> GPLGSEILRHSMDPATFTFNFNNEPWVRGRHETYLCYEVERMHNDTWVKLAQRRGFLANQAKHKHGFLEGRHAALCFLDVIPFWKLDLDQDYRVTCFTSWSPCFSCAQEMAKFISKNKHVSLCIKTARIYDDKGRAAEGLRTLAEAGAKISIMTYSEFKHCWDTFVDHQGAPFQPWDGLDEHSQDLSGRLRAILQNQEN

APOBEC3G (A3G) restricts human immunodeficiency virus type 1 (HIV-1), a finding that prompted extensive studies of APOBEC3 protein restriction of retroviruses and retrotransposons. The APOBEC3 proteins catalyze the deamination of deoxy-cytidine introducing C-to-U modifications in newly synthesized (−)DNA strands of the virus genome, which results in G-to-A mutations in (+)DNA as U is used as a template during (+)DNA strand synthesis. The C-terminal domain (CTD) of these APOBEC3 proteins is catalytically active, containing Zn2+-binding motif HxE-x23–28-C-x2–4-C. The catalytic mechanism of cytosine/cytidine deamination has been studied biochemically and structurally using deaminases from Escherichia coli and yeast. Although all APOBEC3 proteins deaminate cytidines in ssDNA, they show differences in preferred hotspot sequences as 5ʹ-CC for A3G and 5ʹ-TC for other A3s (A3A can deaminate 5ʹ-CC albeit to a lesser extent).

In this study, we present the co-crystal structure of the A3G-CTD and ssDNA at 1.86 Å resolution. Those lysine substitutions were combined with the other three substitutions, which we previously showed to increase catalytic activity. This variant, hereafter called CTD2, spans residues 191–384 of A3G, and contains P200A, L234K, N236A, C243A, P247K, F310K, Q318K, C321A, Q322A, and C356A substitutions. The catalytically inactive CTD2 (CTD2*) was co-crystallized with the 9nt ssDNA containing a 5ʹ-TCCCA target sequence (5ʹ-AATCCCAAA). The interface between protein and ssDNA involves all five nucleotides of the 5′-TCCCA target sequence, and approximately 800 Å2 of surface area on ssDNA is buried in the interface with CTD2*. Overall, CTD2* recognizes 5ʹ-C−2C−1C0 through hydrogen-bonds formed with their Watson–Crick faces, and T−3 and A+1 by using strong π–π interactions. The most remarkable interaction involving T−3 is the π–π stacking with W211. The C2 carbonyl group forms a hydrogen bond with the mainchain amino proton of D317, the N3 atom forms a hydrogen bond with the mainchain amino proton of Q318K, and the amino group forms a hydrogen bond with the sidechain carboxyl group of D316. The target cytosine (C0) is tightly packed under the Zn2+ ion by stacking aromatic rings with the Zn2+-chelating residue H257 and forming a T-shaped π–π interaction with Y315. Since histidine forms stronger π–π stacking with a purine ring than with a pyrimidine ring, this interaction selects purines in the +1 position rather than pyrimidines, providing an explanation for why 5ʹ-CCCA is the preferential deamination sequence. Loop1 migrates toward loop7 upon ssDNA binding, with W211 demonstrating the biggest change with its Cα atom moved by 3.9 Å from the position found in the apo-form CTD-2K3A.> ANIVGGIEYSINNASLCSVGFSVTRGATKGFVTAGHCGTVNATARIGGAVVGTFAARVFPGNDRAWVSLTSAQTLLPRVANGSSFVTVRGSTEAAVGAAVCRSGRTTGYQCGTITAKNVTANYAEGAVRGLTQGNACAGRGDSGGS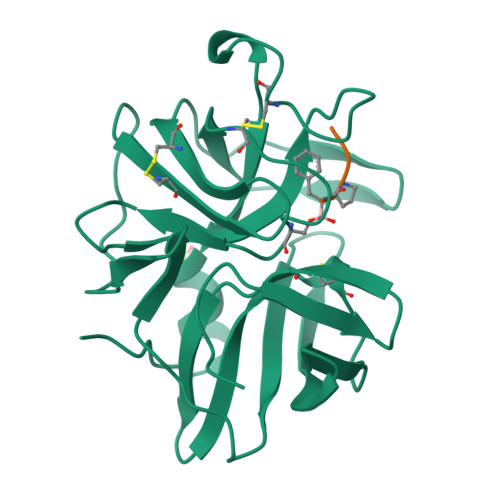WITSAGQAQGVMSGGNVQSNGNNCGIPASQRSSLFERLQPILSQYGLSLVTG;> XAAPF phenylmethanol 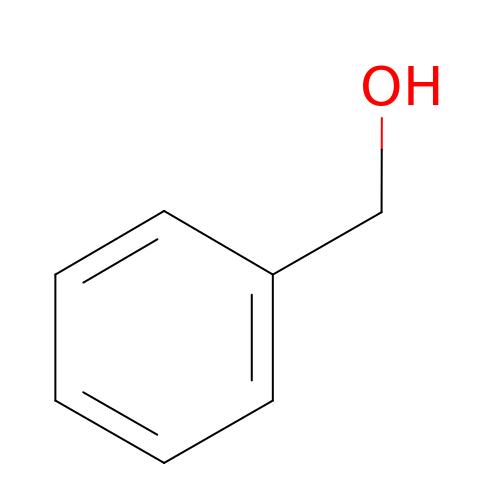| C7 H8 O | WVDDGKGOMKODPV-UHFFFAOYSA-N>[18x]MATYKTPGVYIEEITKFPPSVAQVETAIPAFIGYTQFARTKPSVDSDDLILKPKRISSLLDFTTYYGGAQNEQGITVKLTDTLIEGAENRTINVPEPTFKSPYLMFYSLQMYFANGGGPCYIVSTGVYDDWSDSETPPTINFSDLESGLAVIRKEDEPTLLLFPDATNLPTDDEFYSLYNSALMQCNDLQDRFTILDTYSDQTYNDGVEDLDPIPALRNGIN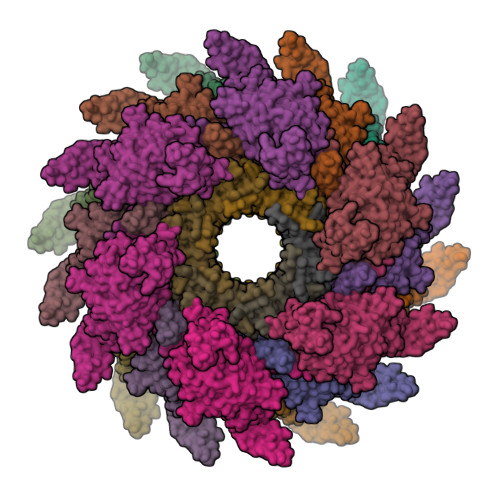LTKDYLKYGAAYYPFVQTILNYQYSADEIVIQHLSYNPNAIATALDNLNAVNGPTFIDAILDDLRDLSLPDISGEISDAVGFMYDDVDGFDIDGTFTTNSVKVANFASLVESVLSTLNELIDAKEEINKDVNSAIASSEEDNAIKTAISDALDVFNEDFEGADKIESVAKNLSDLLIKIKQADTNTKVENVLSINALNFSAEFEKLLTYDVNTGLTASVTLDLFANIGTRLDDIIAAVSAAEPIDVNNGKLNGRLLSDIEPLDNATYNTILLEINSHKVTLPPSSSMAGAYARVDNDRGVWKSPANIGLNYVSKPSVTVSHEEQESMNVHGTGKSVNAIRSFVGKGTLVWGARTLAGNDNEWRYISVRRFFNMAEESIKKATEQFVFEPNDGNTWVRVRAMIENFLILQWRAGALAGAKPEHAFYVKVGLGQTMTAQDILEGNMNVEIGLAVVRPAEFIILKFSHKMQES;>MSYPLSKFHFSVEWGGTKIGFTEVSGLDLETEIIEYRHGASPEYSKIKMPGMQKFSNITLKRGTFKSDNEYFQWYNTINLNKVERRDLTISLLNEEHEPVVTWKVKNAWPLKVQSTDLKGDGNEVAIESMELAHEGLVIQNE[18x]>MRGSHHHHHHGSAERMLATIMFTDIVGSTQHAAALGDDRWRDLLDNHDTIVCHEIQRFGGREVNTAGDGFVATFTSPSAAIACADDIVDAVAALGIEVRIGIHAGEVEVRDASHGTDVAGVAVHIGARVCALAGPSEVLVSSTVRDIVAGSRHRFA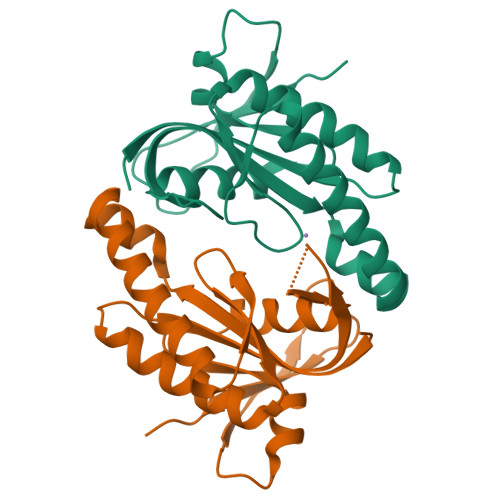ERGEQELKGVPGRWRLCVLMRDDATRTR[4x]> MHHHHHHELENYEQPVVLREDNRRRRRRMKPRSTAASLSSMELIPIEFVLPTSQRNTKTPETALLHVAGHGNVEQMKAQVWLRALETSVSADFYHRLGPDHFLLLYQKKGQWYEIYDKYQVVQTLDCLRYWKVLHRSPGQIHVVQRHAPSEETLAFQRQLNALIGYDVTDVSNVHDDELEFTRRRLVTPRMAEVAGRDPKLYAMHPWVTSKPLPEYLLKKITNNCVFIVIHRSTTSQTIKVSADDTPGTILQSFFTKMAKKKSLMDIPESQNERDFVLRVCGRDEYLVGETPIKNFQWVRQCLKNGEEIHLVLDTPPDPALDEVRKEEWPLVDDCTGVTGYHEQLTIHGKDHESVFTVSLWDCDRKFRVKIRGIDIPVLPRTADLTVFVEANIQYGQQVLCQRRTSPKPFTEEVLWNVWLEFSIKIKDLPKGALLNLQIYCGKAPALSGKTSAEMPSPESKGKAQLLYYVNLLLIDHRFLLRHGEYVLHMWQLSGKGEDQGSFNADKLTSATNPDKENSMSISILLDNYCHPIALPKHRPTPDPEGDRVRAEMPNQLRKQLEAIIATDPLNPLTAEDKELLWHFRYESLKDPKAYPKLFSSVKWGQQEIVAKTYQLLAKREVWDQSALDVGLTMQLLDCNFSDENVRAIAVQKLESLEDDDVLHYLLQLVQAVKFEPYHDSALARFLLKRGLRNKRIGHFLFWFLRSEIAQSRHYQQRFAVILEAYLRGCGTAMLHDFTQQVQVIDMLQKVTIDIKSLSAEKYDVSSQVISQLKQKLENLQNLNLPQSFRVPYDPGLKAGALVIEKCKVMASKKKPLWLEFKCADPTALSNETIGIIFKHGDDLRQDMLILQIL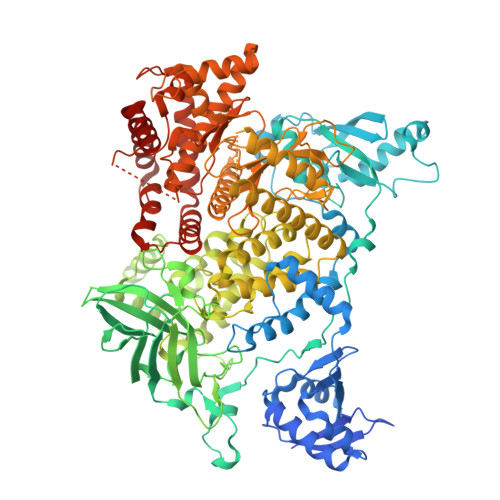RIMESIWETESLDLCLLPYGCISTGDKIGMIEIVKDATTIAKIQQSTVGNTGAFKDEVLSHWLKEKCPIEEKFQAAVERFVYSCAGYCVATFVLGIGDRHNDNIMISETGNLFHIDFGHILGNYKSFLGINKERVPFVLTPDFLFVMGTSGKKTSLHFQKFQDVCVKAYLALRHHTNLLIILFSMMLMTGMPQLTSKEDIEYIRDALTVGKSEEDAKKYFLDQIEVCRDKGWTVQFNWFLHLVLGIKQGEKHSA>[4x]MAQILPIRFQEHLQLQNLGINPANIGFSTLTMESDKFICIREKVGEQAQVVIIDMNDPSNPIRRPISADSAIMNPASKVIALKAGKTLQIFNIEMKSKMKAHTMTDDVTFWKWISLNTVALVTDNAVYHWSMEGESQPVKMFDRHSSLAGCQIINYRTDAKQKWLLLTGISAQQNRVVGAMQLYSVDRKVSQPIEGHAASFAQFKMEGNAEESTLFCFAVRGQAGGKLHIIEVGTPPTGNQPFPKKAVDVFFPPEAQNDFPVAMQISEKHDVVFLITKYGYI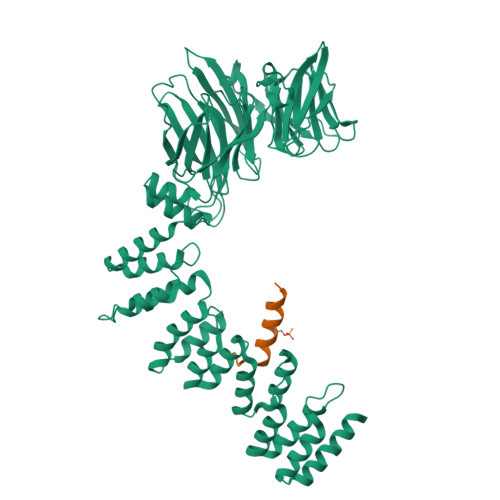HLYDLETGTCIYMNRISGETIFVTAPHEATAGIIGVNRKGQVLSVCVEEENIIPYITNVLQNPDLALRMAVRNNLAGAEELFARKFNALFAQGNYSEAAKVAANAPKGILRTPDTIRRFQSVPAQPGQTSPLLQYFGILLDQGQLNKYESLELCRPVLQQGRKQLLEKWLKEDKLECSEELGDLVKSVDPTLALSVYLRANVPNKVIQCFAETGQVQKIVLYAKKVGYTPDWIFLLRNVMRISPDQGQQFAQMLVQDEEPLADITQIVDVFMEYNLIQQCTAFLLDALKNNR;>[4x]KESALRKQSLYLKFDPLL>[4x]MSLIERVRTDLYRIPLPTRLTDSTHGAMMDFELITVRIEDSDGATGLGYTYTVNHGGAAVATMVDKDLRGCLLGADAEQIEKIWQSMWWRLHYAGRGGHATSAISAVDIALWDLKGIRARTPLWKLFGGYDPVVPVYAGGIDLELPVADLKTQADRFLAGGFRAIKMKVG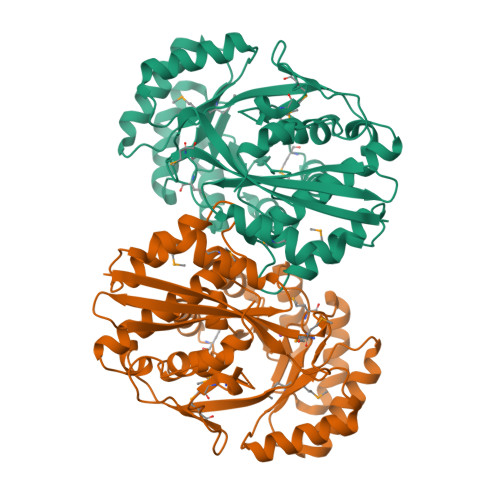RPDLKEDVDRVSALREHLGDSFPLMVDANMKWTVDGAIRAARALAPFDLHWIEEPTIPDDLVGNARIVRESGHTIAGGENLHTLYDFHNAVRAGSLTLPEPDVSNIGGYTTFRKVAALAEANNMLLTSHGVHDLTVHALASVPHRTYMEAHGFGLHAYMAEPMAVTDGCVSAPDRPGHGVVLDFERLGRLAVGEGHHHHHH4,4'-[heptane-1,7-diylbis(oxy)]dibenzenecarboximidamide | C21 H28 N4 O2 | 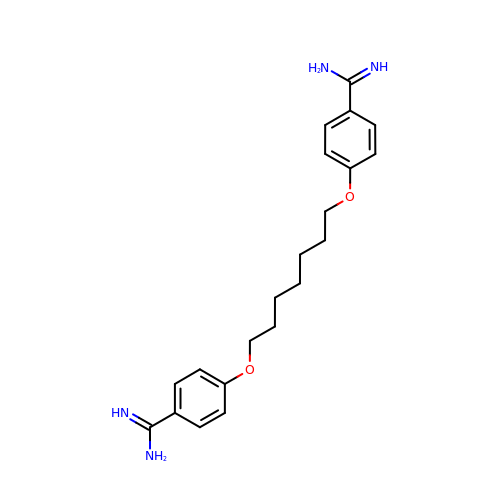IUJKKCRARYRWFG-UHFFFAOYSA-N> MKHHHHHHPMGSELTEAEKRRLLRERRQKKFSNGGASSRLNKI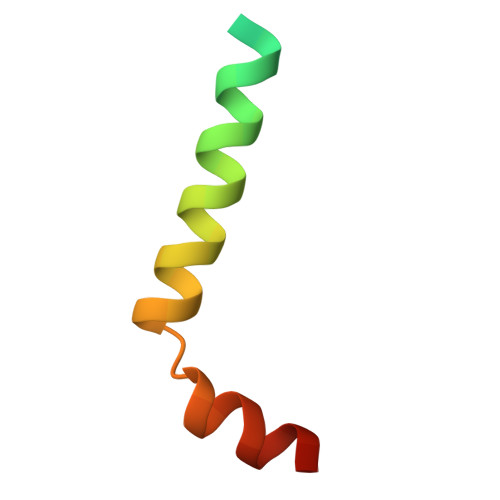TGW>RDSGTVWGALGHGINLNIPNFQMTDDIDEVRWERGSTLVAEFKRKPFLKSGAFEILANGDLKIKNLTRDDSGTYNVTVYSTNGTRILDKAL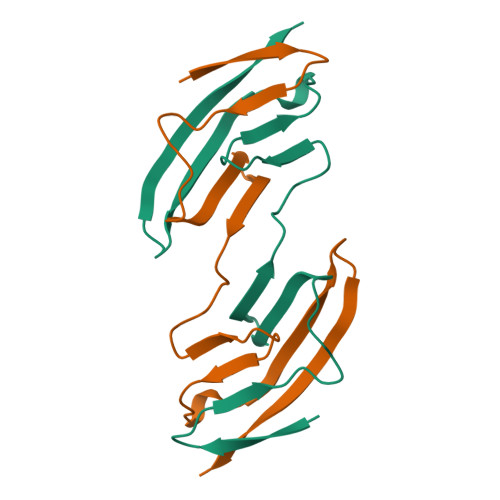DLRILE[2x]>GSNFKAVIKEVRLKSEHGYTNNFPSGDTLFIELDVEAKEDLQDVVAGILIRDRFGQDIFGINTYLMEKKVELKKGKYLFTFKMPLNLAPGKYTLTVALHKGMDHAQECYHWIDNVCNFEV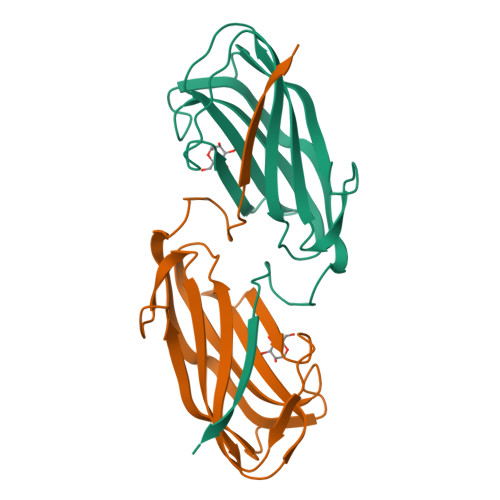NGFKKEQFVGVCYLPTEFNYRKIP[2x]> MTSRDQPRPKGPPKSTSPCPGISNSESSPTLNYQGILNRLKQFPRFSPHFAAELESIYYSLHKIQQDVAEHHKQIGNVLQIVESCSQLQGFQSEEVSPAEPASPGTPQQVKDKTLQESSFEDIMATRSSDWLRRPLGEDNQPETQLFWDKEPWFWHDTLTEQLWRIFAGVHDEKAKPRDRQQAPGLGQESKAPGSCDPGTDPCPEDASTPRPPEASSSPPEGSQDRNTSWGVVQEPPGRASRFLQSISWDPEDFEDAWKRPDALPGQSKRLAVPCKLEKMRILAHGELVLATAISSFTRHVFTCGRRGIKVWSLTGQVAE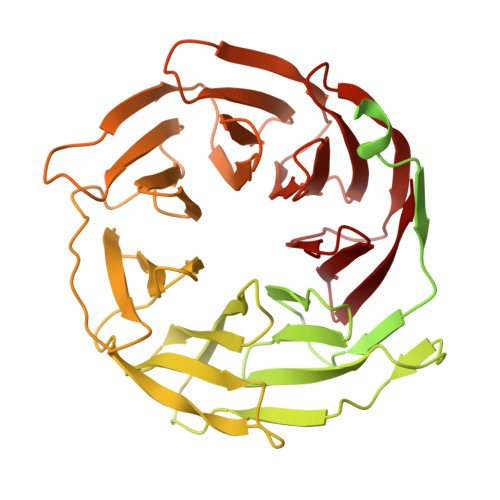DRFPESHLPIQTPGAFLRTCLLSSNSRSLLTGGYNLASVSVWDLAAPSLHVKEQLPCAGLNCQALDANLDANLAFASFTSGVVRIWDLRDQSVVRDLKGYPDGVKSIVVKGYNIWTGGPDACLRCWDQRTIMKPLEYQFKSQIMSLSHSPQEDWVLLGMANGQQWLQSTSGSQRHMVGQKDSVILSVKFSPFGQWWASVGMDDFLGVYSMPAGTKVFEVPEMSPVTCCDVSSNNRLVVTGSGEHASVYQITY The Domain of Unknown Function 26 (DUF26; Gnk2 or stress-antifungal domain; PF01657)18,19 is an extracellular domain harboring a conserved cysteine motif (C-8X-C-2X-C) in its core. The third class of DUF26 domain-containing proteins is the PLASMODESMATA-LOCALIZED PROTEINS (PDLPs). PDLPs contain two DUF26 domains in their extracellular region and a transmembrane helix, but lack a kinase domain. We defined the structural relationship of tandem DUF26 domains by determining crystal structures of AtPDLP5 (residues 26–241) and AtPDLP8 (21–253) ectodomains to 1.25 and 1.95 Å resolution, respectively.

The DUF26-A and B domains in PDLP5 and 8 closely align, with root mean square deviations (r.m.s.d.s) of 1.6 and 1.2 Å when comparing 89 corresponding Cα atoms, respectively. The DUF26-A and -B domains in PDLP5 and PDLP8 have 24% and 30% of their residues in common, most of which map to the hydrophobic core of the domain (including the six cysteine residues forming intra-molecular disulfide bonds) and to the DUF26-A–DUF26-B interface. Consistently, the ectodomains of PDLP5 and PDLP8 belonging to different phylogenetic clades closely align with an r.m.s.d. of ~1.6 Å when comparing 198 corresponding Cα atoms. These observations suggest that evolutionarily distant DUF26 tandem proteins likely share the conserved three-dimensional structure. Notably, Glu130 and Arg132 implicated in mannose binding in Gnk2 are replaced by Asp131 and Lys133 in the DUF-A of PDLP5, respectively. A similar pocket is found in the DUF-A domain of PDLP8, but not in the DUF-B domains of either PDLP5 or 8. We next explored potential binding sites in the two molecules by analyzing sitewise ω for orthologs of PDLP5 and PDLP8. Low ω values were observed in structural context, indicating conservation of residues buried inside the DUF26 domain, while variable residues (under more relaxed selection) appear on the surface of the structure. The different surface charge properties of related PDLPs from Arabidopsis suggest that different PDLPs and other DUF26-containing proteins sense a diverse set of ligands. Notably, we observed typical lectin-dimers in PDLP5 and PDLP8 crystals, in which two lectin domains dimerized along an extended antiparallel β-sheet.

>[3x]SSSESHIFIYGGCSPEKYTPNTPFESNRDTFLSSVVTSSSDASFNSFAVGNDSSSSSSSSAVFGLYQCRDDLRSSDCSKCIQTSVDQITLICPYSYGASLQLEGCFLRYETNDFLGKPDTSLRYKKCSSKSVENDYDFFKRRDDVLSDLESTQLGYKVSRSGLVEGYAQCVGDLSPSDCTACLAESVGKLKNLCGSAVAAEVYLAQCYARYWGSGYYDFSSDPTNGDHVGKSLEGSENLYFQ>[4x]GAGAGAGAGAGMFRLTRLSNKPILSPIKEHEWEKEAVFNAAVIYEGNKFHLFYRASNNKFVLNTEKPEEKYKFVSSIGYAVSEDGINFERFDKPVLVGEIPQEAWGVEDPRITKIDNKYYMLYTGFGGRDWLDFRICMVWSDDLKNWKGHRIVLDEPNKDAALLSEKIN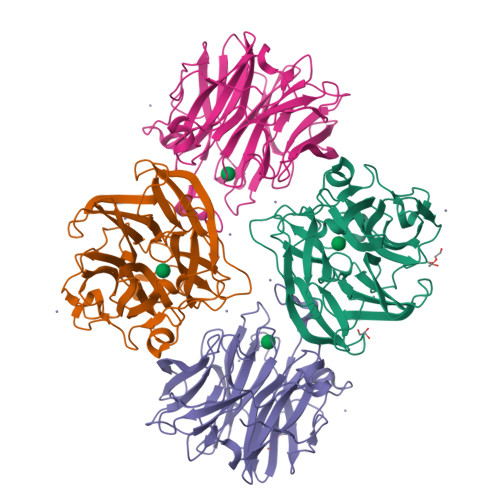GKYVLFHRRMPDIWIAYSDDLVNWYNHKIIMSPKSHTWESKKIGIAGPPIKREDGWLLIYHGVDNNNVYRLGVALLDLKDPSKVIARQKEPILEPELDWEINGLVPNVVFSCGAVEVNDMYYVYYGAADTHIGVAVIEKEKVKF> MPDQRQTRFAHITKAHPCFNEKLHDRVGRVHVPIAPRCNIHCKFCTRDINECERRPGVTGRLMTADDAIKHVEKVKEEM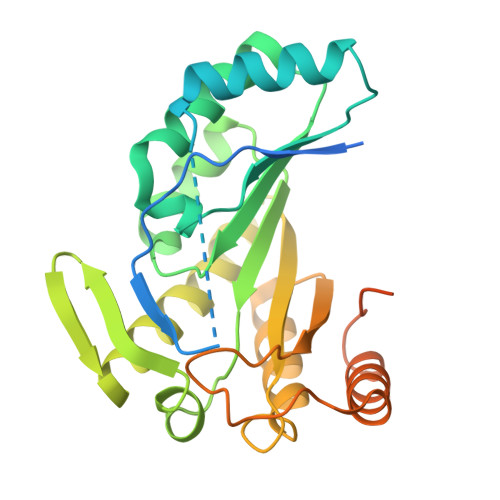PISVIGVAGPGDALANEETFEFFKKASKKFPDLLKCMSTNGLLLPDRADELAELGINTVTVTVNAVDPEIGEKIYSFVVYKDKVYHGREAFEVLSRNQLEGIEKLAERGIIVKVNSVLIPGLNDEHIVDIAREVKKRGASLMNIIPLIPMGEMKDYPRPTCEQIERVRNEVEKIIPVFRACTQCRADAYGIPGKKEADKHLDMTPASHYLEHHHHHH N-cyclohexyl-D-leucyl-N-[(1-aminoisoquinolin-6-yl)methyl]-4,4-difluoro-L-prolinamide | C27 H37 F2 N5 O2 | 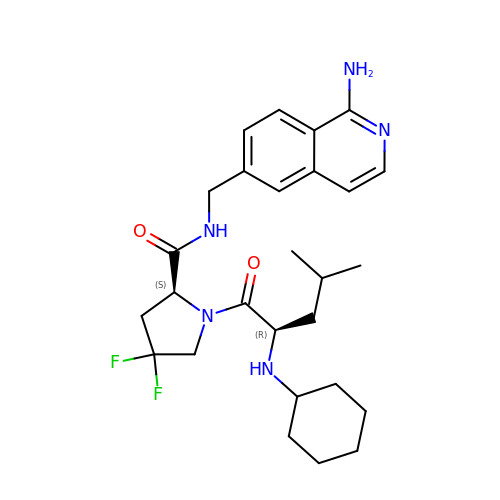COYOMWYNPNKVLE-PKTZIBPZSA-N> SKFLDRFRYAKQKGETFADGHGQLLNTNRDWEDGYRQRWQHDKIVRSTHGVNCTGSCSWKIYVKNGLVTWETQQTDYPRTRPDLPNHEPRGCPRGASYSWYLYSANRLKYPMMRKRLMKMWREAKALHSDPVEAWASIIEDADKAKSFKQARGRGGFVRSSWQEVNELIAASNVYTIKNYGPDRVAGFSPIPAMSMVSYASGARYLSLIGGTCLSFYDWYCDLPPASPQTWGEQTDVPESADWYNSSYIIAWGSNVPQTRTPDAHFFTEVRYKGTKTVAVTPDYAEIAKLCDLWLAPKQGTDAAMALAMGHVMLREFHLDNPSQYFTDYVRRYTDMPMLVMLEERDGYYAAGRMLRAADLVAALGQENNPEWKTVAFNTNGEMVAPNGSIGFRWGEKGKWNLEQRDGKTGEETELQLSLLGSQDEIAEVGFPYFGGDGTEHFNKVELENVLLHKLPVKRLQLADGSTALVTTVYDLTLANYGLERGLNDVNCATSYDDVKAYTPAWAEQITGVSRSQIIRIAREFADNADKTHGRSMIIVGAGLNHWYHLDMNYRGLINMLIFCGCVGQSGGGWAHYVGQEKLRPQTGWQPLAFALDWQRPARHMNSTSYFYNHSSQWRYETVTAEELLSPMADKSRYTGHLIDFNVRAERMGWLPSAPQLGTNPLTIAGEAEKAGMNPVDYTVKSLKEGSIRFAAEQPENGKNHPRNLFIWRSNLLGSSGKGHEFMLKYLLGTEHGIQGKDLGQQGGVKPEEVDWQDNGLEGKLDLVVTLDFRLSSTCLYSDIILPTATWYEKDDMNTSDMHPFIHPLSAAVDPAWEAKSDWEIYKAIAKKFSEVCVGHLGKETDIVTLPIQHDSAAELAQPLDVKDWKKGECDLIPGKTAPHIMVVERDYPATYERFTSIGPLMEKIGNGGKGIAWNTQSEMDLLRKLNYTKAEGPAKGQPMLNTAIDAAEMILTLAPETNGQVAVKAWAALSEFTGRDHTHLALNKEDEKIRFRDIQAQPRKIISSPTWSGLEDEHVSYNAGYTNVHELIPWRTLSGRQQLYQDHQWMRDFGESLLVYRPPIDTRSVKEVIGQKSNGNQEKALNFLTPHQKWGIHSTYSDNLLMLTLGRGGPVVWLSEADAKDLGIADNDWIEVFNSNGALTARAVVSQRVPAGMTMMYHAQERIVNLPGSEITQQRGGIHNSVTRITPKPTHMIGGYAHLAYGFNYYGTVGSNRDEFVVVRKMKNIDWLDGEGNDQVQES;> MKIRSQVGMVLNLDKAIGCHTCSVTCKNVWTSREGVEYAWFNNVETKPGQGFPTDWENQEKYKGGWIRKINGKLQPRMGNRAMLLGKIFANPHLPGIDDYYEPFDFDYQNLHTAPEGSKSQPIARPRSLITGERMAKIEKGPNWEDDLGGEFDKLAKDKNFDNIQKAMYSQFENTFMMYLPRLCEHCLNPACVATCPSGAIYKREEDGIVLIDQDKCRGWRMCITGCPYKKIYFNWKSGKSEKCIFCYPRIEAGQPTVCSETCVGRIRYLGVLLYDADAIERAASTENEKDLYQRQLDVFLDPNDPKVIEQAIKDGIPLSVIEAAQQSPVYKMAMEWKLALPLHPEYRTLPMVWYVPPLSPIQSAADAGELGSNGILPDVESLRIPVQYLANLLTAGDTKPVLRALKRMLAMRHYKRAETVDGKVDTRALEEVGLTEAQAQEMYRYLAIANYEDRFV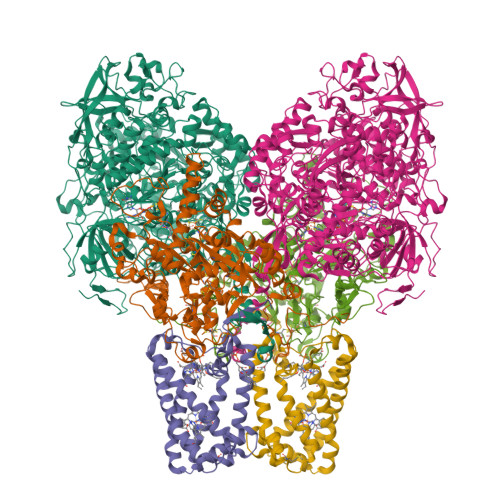VPSSHRELAREAFPEKNGCGFTFGDGCHGSDTKFNLFNSRRIDAIDVTSKTE;> MQFLNMFFFDIYPYIAGAVFLIGSWLRYDYGQYTWRAASSQMLDRKGMNLASNLFHIGILGIFVGHFFGMLTPHWMAAAWLPIEVKQKMAMFAGGASGVLCLIGGVLLLKRRLFSPRVRATTTGADILILSLLVIQCALGLLTIPFSAQHMDGSEMMKLVGWAQSVVTFHGGASQHLDGVAFIFRLHLVLGMTLFLLFPFSRLIHIWSVPVEYLTRKYQLVRARH> MFCFSRGLWMRHIGQDVPKRHTHFVLESRLMYEKSFRDCWLHSVCRAISQLDEPLSKTVVGTHQKMLQRKVTCFQ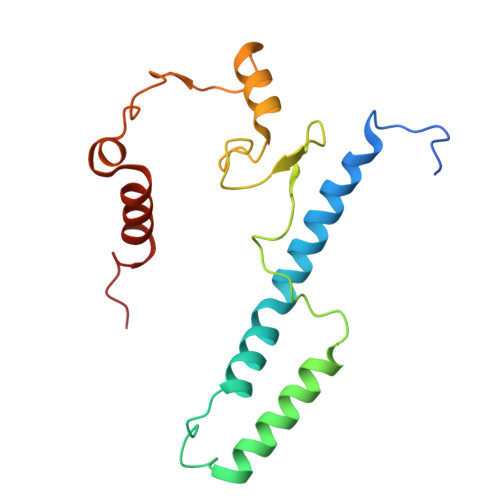YNQYGLFKTPYYRLANVDRYHAVQGVAGTREWVPYVNVSYWTMNKMVRGGNLLVHRVHYTGWGTDSHLKKGGWEHRWNKVLQRNVLQYSRI> SSLDDKPQFPGASAEFIDKLEFIQPNVISGIPIYRVMDRQGQIINPSEDPHLPKEKVLKLYKSMTLLNTMDRILYESQRQGRISFYMTNYGEEGTHVGSAAALDNTDLVFGQYREAGVLMYRDYPLELFMAQCYGNISDLGKGRQMPVHYGCKERHFVTISSPLATQIPQAVGAAYAAKRANANRVVICYFGEGAASEGDAHAGFNFAATLECPIIFFCRNNGYAISTPTSEQYRGDGIAARGPGYGIMSIRVDGNDVFAVYNATKEARRRAVAENQPFLIEAMTYRIGHHDTSDDSSAYRSVDEVNYWDKQDHPISRLRHYLLSQGWWDEEQEKAWRKQSRRKVMEAFEQAERKPKPNPNLLFSDVYQEMPAQLRKQQESLARHLQTYGEHYPLDHFDK;> VAHFTFQPDPEPREYGQTQKMNLFQSVTSALDNSLAKDPTAVIFGEDVAFGGVFRCTVGLRDKYGKDRVFNTPLCEQGIVGFGIGIAVTGATAIAEIQFADYIFPAFDQIVNEAAKYRYRSGDLFNCGSLTIRSPWGCVGHGALYHSQSPEAFFAHCPGIKVVIPRSPFQAKGLLLSCIEDKNPCIFFEPKI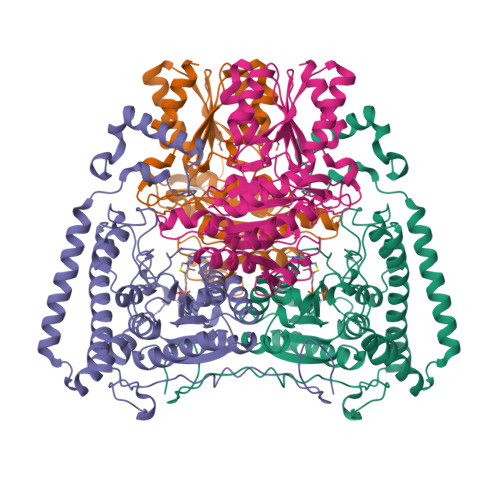LYRAAAEEVPIEPYNIPLSQAEVIQEGSDVTLVAWGTQVHVIREVASMAKEKLGVSCEVIDLRTIIPWDVDTICKSVIKTGRLLISHEAPLTGGFASEISSTVQEECFLNLEAPISRVCGYDTPFPHIFEPFYIPDKWKCYDALRKMINY> MANELTWHDVLAEEKQQPYFLNTLQTVASERQSGVTIYPPQKDVFNAFRFTELGDVKVVILGQDPYHGPGQAHGLAFSVRPGIAIPPSLLNMYKELENTIPGFTRPNHGYLESWARQGVLLLNTVLTVRAGQAHSHASLGWETFTDKVISLINQHREGVVFLLWGSHAQKKGAIIDKQRHHVLKAPHPSPLSAHRG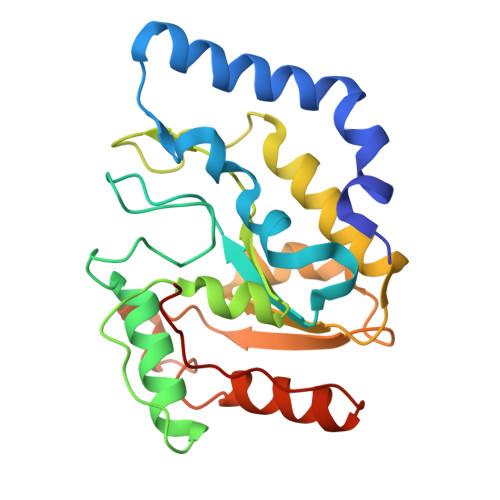FFGCNHFVLANQWLEQRGETPIDWMPVLPAESE>SNARRGPAGIGRTGRGMGGLFSVGETTAKVLKDEIDVKFKDVAGCEEAKLEIMEFVNFLKNPKQYQDLGAKIPKGAILTGPPGTGKTLLAKATAGEANVPFITVSGSEFLEMFVGVGPARVRDLFALARKNAPCILFIDQIDAVGRKRGRGNFGGQSEQENTLNQLLVEMDGFNTTTNVVILAGTNRPDILDPALLRPGRFDR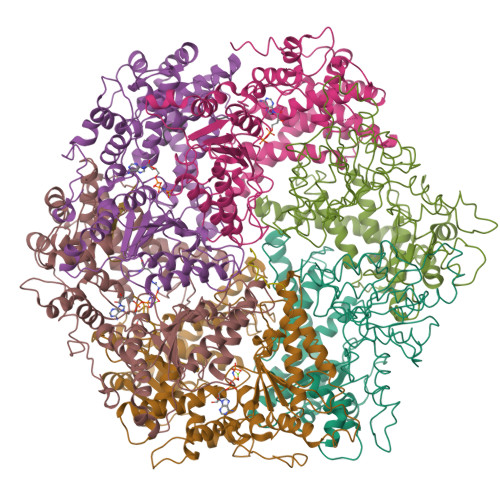QIFIGPPDIKGRASIFKVHLRPLKLDSTLEKDKLARKLASLTPGFSGADVANVCNEAALIAARHLSDSINQKHFEQAIERVIGGLEKKTQVLQPEEKKTVAYHQAGHAVAGWYLEHADPLLKVSIIPRGKGLGYAQYLPKEQYLYTKEQLLDRMCMTLGGRVSEEIFFGRITTGAQDDLRKVTQSAYAQIVQFGMNEKVGQISFDLPRQGDMVLEKPYSEATARLIDDEVRILINDAYKRTVALLTEKKADVEKVALLLLEKEVLDKNDMVELLGPRPFAEKSTYEEFVEGTGSLDEDTSLPEGLKDWNKEREKEKEEPPGEKVAN[6x];>[4x]AAAAAAAAAAA6-[BIS(2,2,2-TRIFLUOROETHYL)AMINO]-4-(TRIFLUOROMETHYL)QUINOLIN-2(1H)-ONE 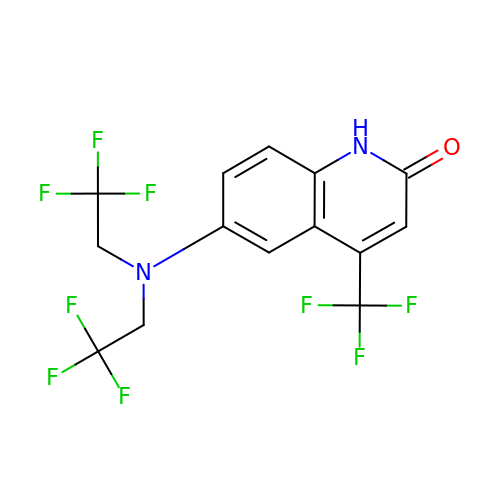| C14 H9 F9 N2 O | ULBPQWIGZUGPHU-UHFFFAOYSA-N>[2x]MKQKPAFIPYAGAQFEPEEMLSKSAEYYQFMDHRRTVREFSNRAIPLEVIENIVMTASTAPSGAHKQPWTFV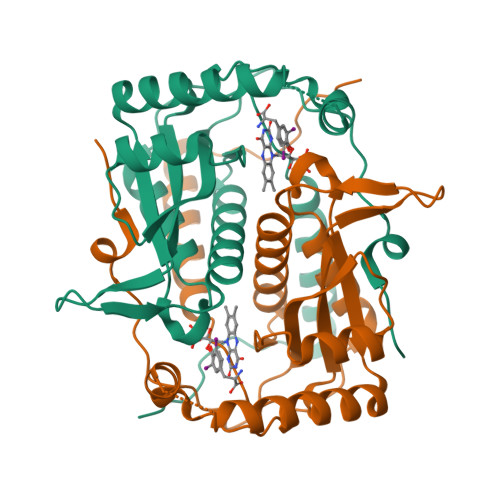VVSDPQIKAKIRQAAEKEEFESYNGRMSNEWLEDLQPFGTDWHKPFLEIAPYLIVVFRKAYDVLPDGTQRKNYYVQESVGIACGFLLAAIHQAGLVALTHTPSPMNFLQKILQRPENERPFLLVPVGYPAEGAMVPDLQRKDKAAVMVVYHHHHHH>ADEPATLRGVSAETEKHISAGKARLQDLRDAERRCHDAWQAIVVIDGGSSATRTNVFLAKTRSCPRGGRHIDPDSIRLLGAGKRFAGLRGVLESWLDAYAGEDWESRSVDSKRLFQHVPEMEDSARGLMQLLEDDAVRILDEKLTEEQKVQVQAMGVPVLLCSTAGVRDFHDWYREALFVILRFLINHPKPGHGYKFFTNPEWTRPITGAEEGLYAFLALNHLSGRLGEDPARCYVDEYGMKQCRNDLVGVVEVGGASTQIVFPLQDGTALPSSIRAVNLQHERFLPSRFPSADVISVSFMQLGVASSSGLFFKELCSNAEFRHQGICYNPCIFRGFRQACSAGDVEILPDGTIVVDEDVRKNKLKPVATYCSANNPEISFKAMNEIQCRVNKIDPTKSLAERLRIDDCFQIVGTGDFDTCQAQVEELLVSPRFPLPANIEAASSGFESVGQVFKFASTASPMVITGGAMYASISTMQGLGLLPKDFQGDLEQLIAASRTYCSSPVVNNGDGLVIQLPNAEQK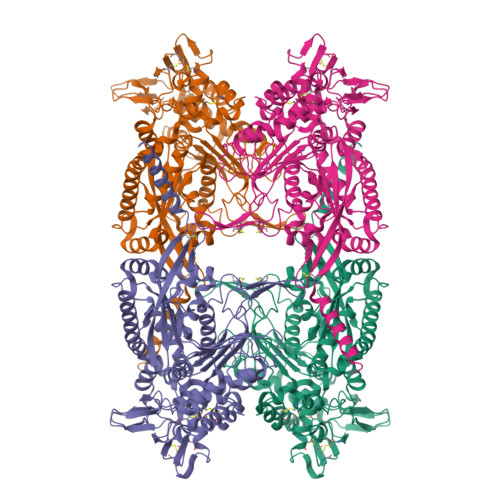LTSMNYDLCKTIALTVSLLQHMEAGEHKPSSISWQKTVVGPDGKPRADLGWHVGAILHRVLFTEEWGRTAYETGFTYNM[2x]benzyl 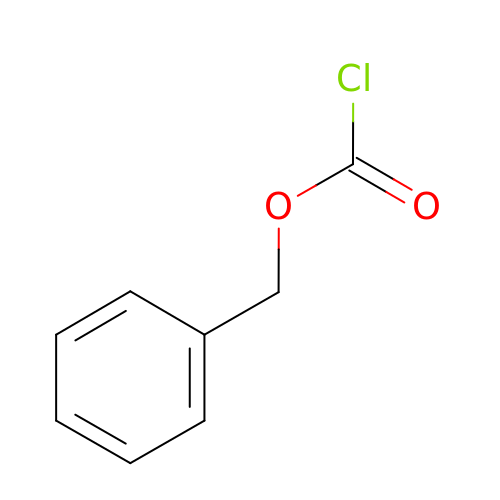chlorocarbonate | C8 H7 Cl O2 | HSDAJNMJOMSNEV-UHFFFAOYSA-N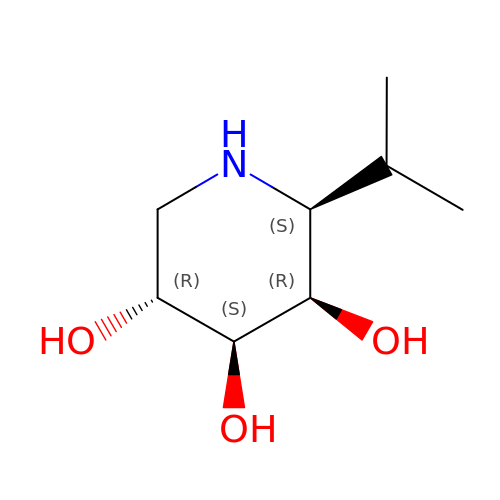(2S,3R,4S,5R)-2-(1-methylethyl)piperidine-3,4,5-triol | C8 H17 N O3 | WNBLNSHOIGFFFW-VGRMVHKJSA-N> PGSMDQTYSLESFLNHVQKRDPNQTEFAQAVREVMTTLWPFLEQNPKYRQMSLLERLVEPERVIQFRVVWVDDRNQVQVNRAWRVQFSSAIGPYKGGMRFHPSVNLSILKFLGFEQTFKNALTTLPMGGGKGGSDFDPKGKSEGEVMRFCQALMTELYRHLGADTDVPAGDIGVGGREVGFMAGMMKKLSNNTACVFTGKGLSFGGSLIRPEATGYGLVYFTEAMLK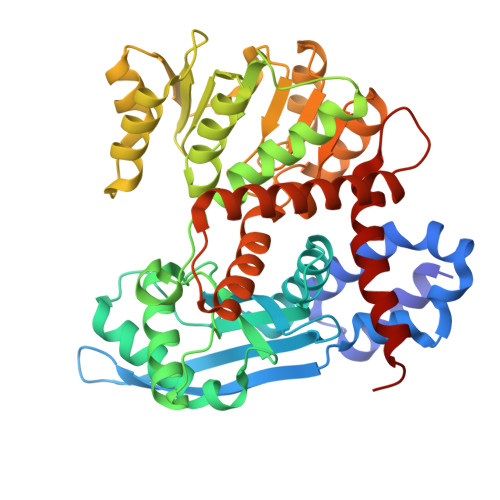RHGMGFEGMRVSVSGSGNVAQYAIEKAMEFGARVITASDSSGTVVDESGFTKEKLARLIEIKSSRDGRVADYAKEFGLVYLEGQQPWSVPVDIALPCATQNELDVDAAHQLIANGVKAVAEGANMPTTIEATELFQQAGVLFAPGKAANAGGVATSGLEMAQNAARLGWKAEKVDARLHHIMLDIHHACVEHGGEGEQTNYVQGANIAGFVKVADAMLAQGVI>[3x]GAMGSLIRKKAAGLESAATIRTKVFVWGLNDKDQLGGLKGSKIKVPSFSETLSALNVVQVAGGSKSLFAVTVEGKVYACGEATNGRLGLGISSGTVPIPRQITALSSYVVKKVAVHSGGRHATALTVDGKVFSWGEGDDGKLGHFSRMNCDKPRLIEALKTKRIRDIACGSSHSAALTSSGELYTWGLGEY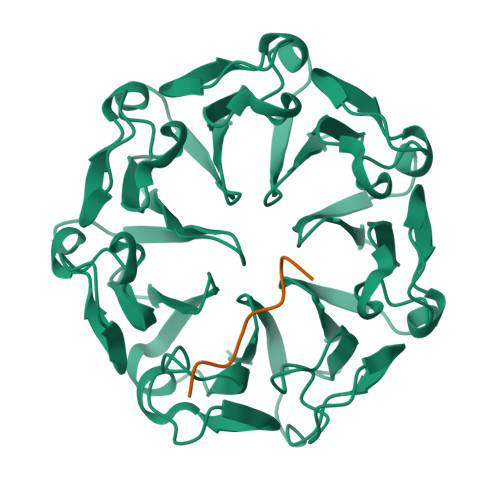GRLGHGDNTTQLKPKMVKVLLGHRVIQVACGSRDAQTLALTDEGLVFSWGDGDFGKLGRGGSEGCNIPQNIERLNGQGVCQIECGAQFSLALTKSGVVWTWGKGDYFRLGHGSDVHVRKPQVVEGLRGKKIVHVAVGALHCLAVTDSGQVYAWGDNDHGQQGNGTTTVNRKPTLVQGLEGQKITRVACGSSHSVAWTTVDVATPSVHEPVLFQT;>[3x]DEDKDKDETETVKQT>[6x]GSHMSQSLFSLAFGVGTQNRQEAWLEVFYALPLLKPSSEIVAAVAPILGYAAGNQALTFTSQQAYQLADALKGIDAAQSALLSRLAESQKPLVATLLAEDAAPSSTAEAYLKLHLLSHRLVKP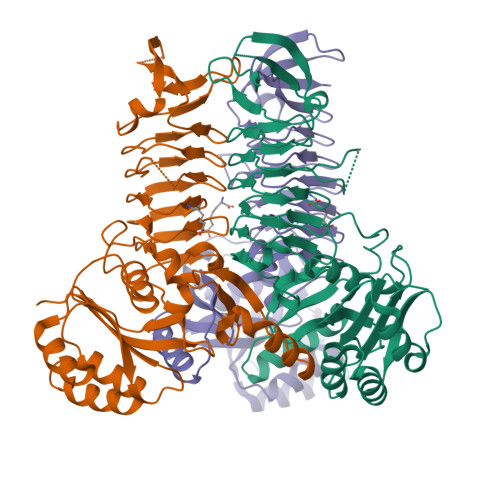HAVNLSGIFPLLPNVAWTNIGAVDLAELAELQLEARLKGKLLEVFSVDKFPKMTDYVVPAGVRIADTARVRLGAYIGEGTTVMHEGFVNFNAGTEGPGMIEGRVSAGVFVGKGSDLGGGCSTMGTLSGGGNIVISVGEGCLIGANAGIGIPLGDRNIVEAGLYITAGTKVALLDEQNALVKVVKARDLAGQPDLLFRRNSQNGAVECKTNKTAIELNEALHAHN> GHMWSATNEEDDLSVEAEIAHQIAESFSKKYKFPSRSSGIFLYNFEQLKMNLDDIVKEAKNVPGVTRLAHDGSKLPLRCVLGWVALANSKKFQLLVEANKLNKIMQDDLNRY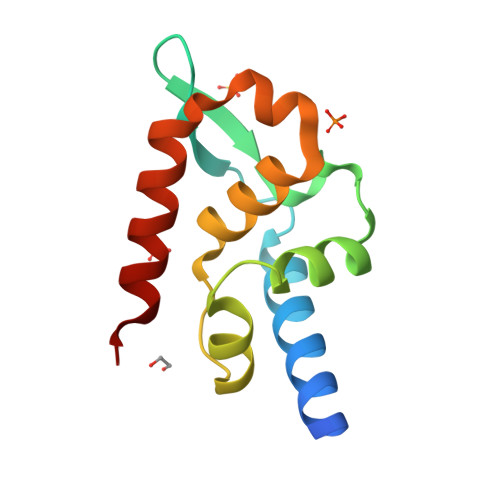ASS> RNSFYMGTCQDEPEQLDDWNRI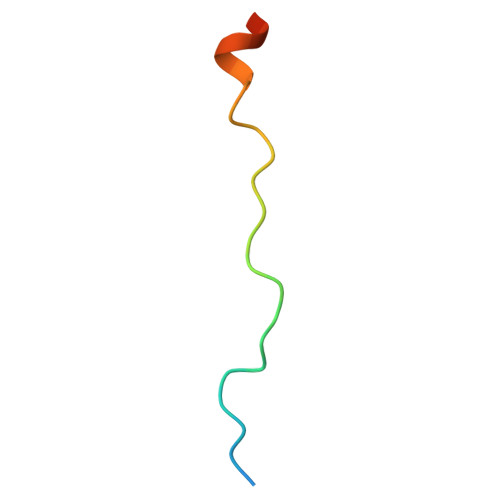AELQQR>[2x]MGMKLLVVSWGDFERWKETKYRFGGETSVGPSTLPILQKVIKPDWTVIVLSDTIGKDFSSVETLREDVRNRVMDFLDRIGAGREVDVIIAPGIGEFTHGSFRGSAMDAYYYVLHALSEII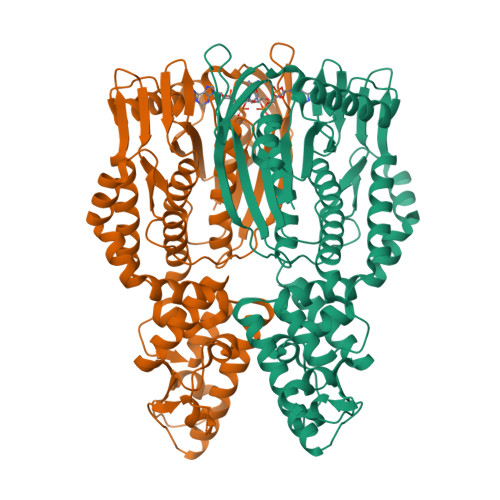PTKGDLEVHFDSTHGLNYVTLLTYRALKDLLGIAAVMNTVTFYAYNSDPFVPKITKELNINTIETTMVKPTPLSEPLPGFDEYLCPYSMERAEFVRLKGSLNTLKNLRKEKKKLEAWIGSLLFGLPLLFLEEFPDIGRLESYIEELAETWGGAIAVNAEEKAVTRRLAFGSGFGTLVKLLFQARITRGLLVEEPYSIEKLYSVSDRLFRGSTLQRVRVELGKIEDKAIKYARKGAFPRDIPLRDFLGFDAANREVSPRNVLAAAGLEANVVEVSMEAWEPKRPEEEAGRHTHLKYTPVGLKKVEDIVSRALKESHHHHHH>[3x]VEADPYEIVIKQLERAAQYMEISEEALEFLKRPQRIVEVTIPVEMDDGSVKVFTGFRVQHNWARGPTKG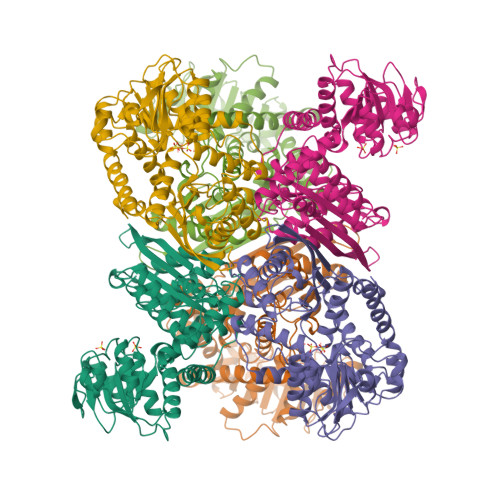GIRWHPEETLSTVKALAAWMTWKTAVMDLPYGGGKGGIIVDPKKLSDREKERLARGYIRAIYDVISPYEDIPAPDVYTNPQIMAWMMDEYETISRRKTPAFGIITGKPLSIGGSLGRIEATARGASYTIREAAKVLGWDTLKGKTIAIQGYGNAGYYLAKIMSEDFGMKVVAVSDSKGGIYNPDGLNADEVLKWKNEHGSVKDFPGATNITNEELLELEVDVLAPAAIEEVITKKNADNIKAKIVAEVANGPVTPEADEILFEKGILQIPDFLCNAGGVTVSYFEWVQNITGYYWTIEEVRERLDKKMTKAFYDVYNIAKEKNIHMRDAAYVVAVQRVYQAMLDRGWVKH> RLGRQALLFPLCLVLYEFSTYIGNDMIQPGMLAVVEQYQAGIDWVPTSMTAYLAGGMFLQWLLGPLSDRIGRRPVMLAGVVWFIVTCLAILLAQNIEQFTLLRFLQGISLCFIGAVGYAAIRESFEEAVCIKITALMANVALIAPLLGPLVGAAWIHVLPWEGMFVLFAALAAISFFGLQRAMP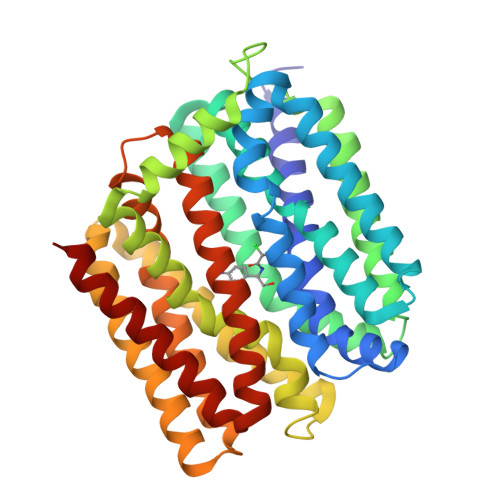ETATRIGEKLSLKELGRDYKLVLKNGRFVAGALALGFVSLPLLAWIAQSPIIIITGEQLSSYEYGLLQVPIFGALIAGNLLLARLTSRRTVRSLIIMGGWPIMIGLLVAAAATVISSHAYLWMTAGLSIYAFGIGLANAGLVRLTLFASDMSKGTVSAAMGMLQMLIFTVGIEISKHAWLNGGNGLFNLFNLVNGILWLSLMVIFLK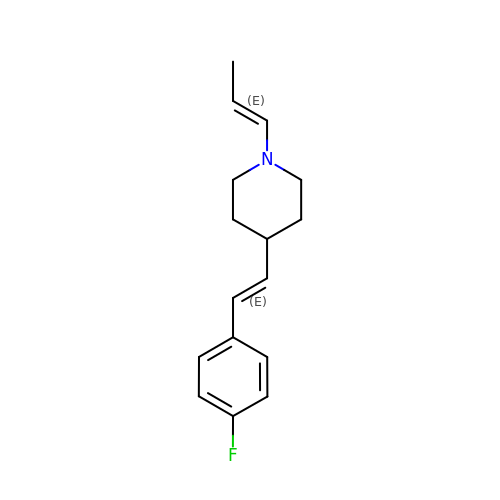4-[(~{E})-2-(4-fluorophenyl)ethenyl]-1-[(~{E})-prop-1-enyl]piperidine | C16 H20 F N | MSBXCAPJLPROOO-FRKQTSRXSA-N>[2x]ATHEVHM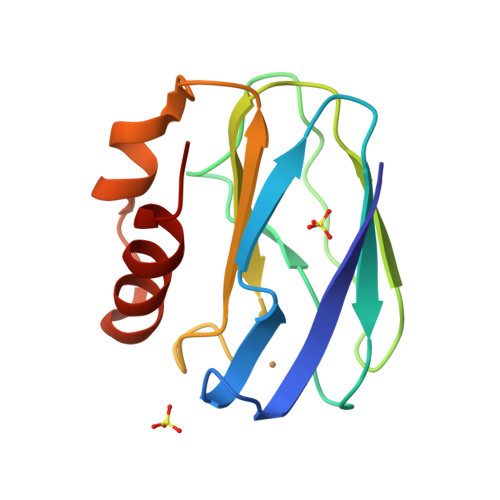LNKGESGAMVFEPAFVRAEPGDVINFVPTDKSHNVEAIKEILPEGVESFKSKINESYTLTVTEPGLYGVKCTPHFGMGMVGLVQVGDAPENLDAAKTAKMPAKARERMDAELAQVN> VPEAPTPMWPDDLQNHTFLHTVYCQDGSPSVGLSEAYDEDQLFFFDFSQNTRVPRLPEFADWAQEQGDAPAILFDKEFCEWMIQQIGPKLDGKIPVSRGFPIAEVFTLKPLEFGKPNTLVCFVSNLFPPMLTVNWQHHSVPVEGFGPTFVSAVDGLSFQAFSYLNFTPEPSDIFSCIVTHEIDRYTAI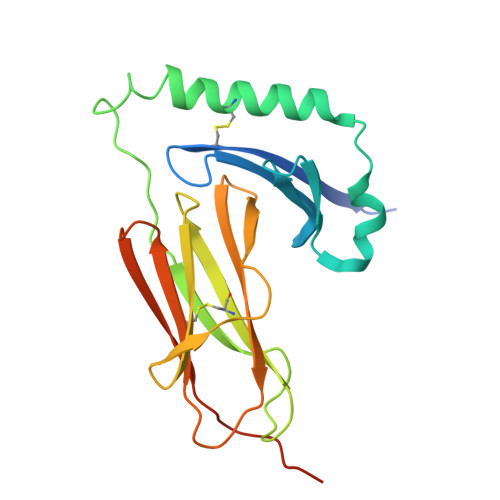AYWVPRNALPSDLLEDYKDDDDK> SRSKVSVAPLHLESAKEPPLNTYKPKEPFTATIVSVESLVGPKAPGETCHIVIDHGGNVPYWEGQSYGVIPPGENPKKPGAPQNVRLYSIASTRYGDNFDGRTGSLCVRRAVYYDPETGKEDPSKNGVCSNFLCNSKPGDKIQLTGPSGKIMLLPEEDPNATHIMIATGTGVAPFRGYLRRMFMEDVPNYRFGGLAWLFLGVANSDSLLYDEEFTSYLKQYPDNFRYDKVLSREQKNRSGGKM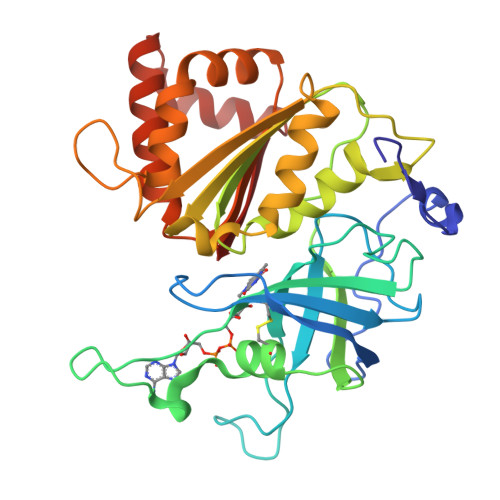YVQDKIEEYSDEIFKLLDGGAHIYFCGLKGMMPGIQDTLKKVAERRGESWDQKLAQLKKNKQWHVEVY> NATQINEELYRLLEDTEILNQEITEGLLKGFEVPDAGVAIQLSKRDVVYPARILIIVLSEMWRFGLTKQSESFLAQVLTTIQKVVTQLKGNDLIPSGVFWLANVRELYSFVVFALNSILTEETFKNGMTDEEYKEYVSLVTELKDDFEALSYNIYNIWLKKLQKQLQKKAINAVVISESLPGFSAGETSGFLNKIFANTEEYTMDDILTFFNSIYWCMKSFH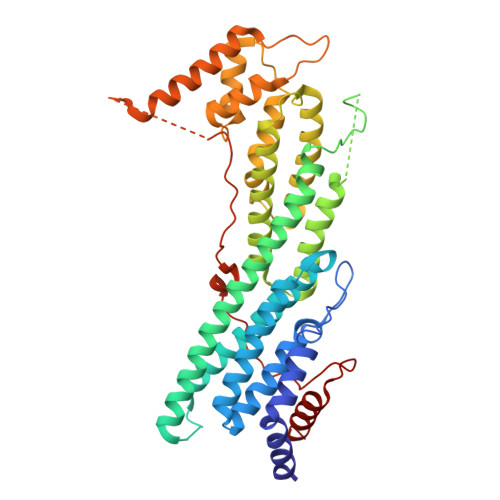IENEVFHAVVTTLLNYVDAICFNELIMKRNFLSWKRGLQLNYNVTRLEEWCKTHGLTDGTECLQHLIQTAKLLQVRKYTIEDIDILRGICYSLTPAQLQKLISQYQVADYESPIPQEILRYVADIVKKEAALSSSGNDSKGHEHSSSIFITPETGPFTDPFSLIKTRKFDQVEAYIPAWLSLPSTKRIVDLVAQQVV> WGSGEVKLRL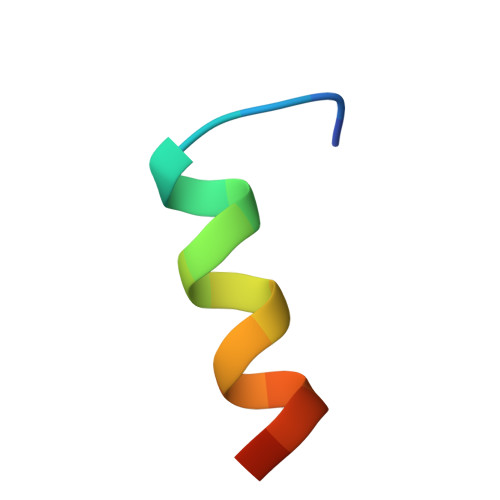QEFLLSKS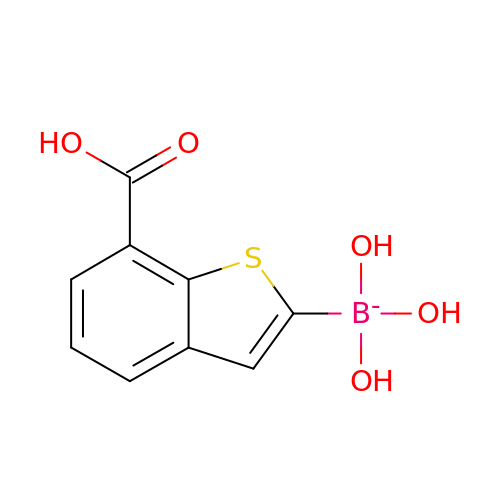(7-carboxy-1-benzothiophen-2-yl)-tris(oxidanyl)boranuide | C9 H8 B O5 S | RPQQLQILJXVZRU-UHFFFAOYSA-N> MFSAGHKIKGTVVLMPKNELEVNPDGSAVDNLNAFLGRSVSLQLISATKADAHGKGKVGKDTFLEGINTSLPTLGAGESAFNIHFEWDGSMGIPGAFYIKNYMQVEFFLKSLTLEAISNQGTIRFVCNSWVYNTKLYKSVRIFFANHTYVPSETPAPLVSYREEELKSLRGNGTGERKEYDRIYDYDVYNDLGNPDKSEKLARPVLGGSSTFPYPRRGRTGRGPTVTDPNTEKQGEVFYVPRDENLGHLKSKDALEIGTKSLSQIVQPAFESAFDLKSTPIEFHSFQDVHDLYEGGIKLPRDVISTIIPLPVIKELYRTDGQHILKFPQPHVVQVSQSAWMTDEEFAREMIAGVNPCVIRGLEEFPPKSNLDPAIYGDQSSKITADSLDLDGYTMDEALGSRRLFMLDYHDIFMPYVRQINQLNSAKTYATRTILFLREDGTLKPVAIELSLPHSAGDLSAAVSQVVLPAKEGVESTIWLLAKAYVIVNDSCYHQLMSHWLNTHAAMEPFVIATHRHLSVLHPIYKLLTPHYRNNMNINALARQSLINANGIIETTFLPSKYSVEMSSAVYKNWVFTDQALPADLIKRGVAIKDPSTPHGVRLLIEDYPYAADGLEIWAAIKTWVQE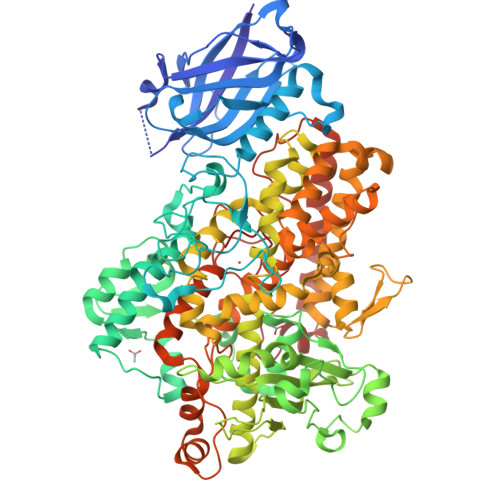YVPLYYARDDDVKNDSELQHWWKEAVEKGHGDLKDKPWWPKLQTLEDLVEVCLIIIWIASALHAAVGFGQYPYGGLIMNRPTASRRLLPEKGTPEYEEMINNHEKAYLRTITSKLPTLISLSVIEILSTHASDEVYLGQRDNPHWTSDSKALQAFQKFGNKLKEIEEKLVRRNNDPSLQGNRLGPVQLPYTLLYPSSEEGLTFRGIPNSISI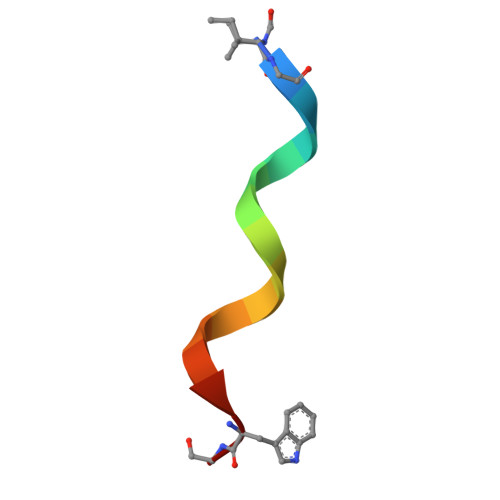> XGALAVVVWLYLWLWX> SMQSSKRSSRSVEDDKEGHLVCRIGDWLQERYEIVGNLGEGTFGKVVECLDHARGKSQVALKIIRNVGKYREAARLEINVLKKIKEKDKENKFLCVLMSDWFNFHGHMCIAFELLGKNTFEFLKENNFQPYPLPHVRHMAYQLCHALRFLHENQLTHTDLKPENILFVNSEFETLYNEHKSCEEKSVKNTSIRVADFGSATFDHEHHTTIVATRHYRPPEVILELGWAQPCDVWSIGCILFEYYRGFTLFQTHENREHLVMMEKILGPIPSHMIHRTRKQKYFYKGGLVWDENSSDGRYVK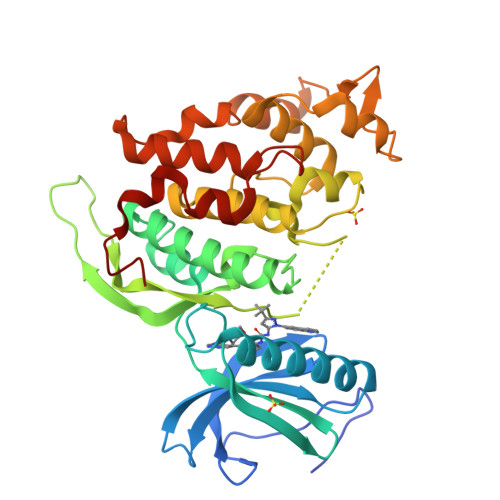ENCKPLKSYMLQDSLEHVQLFDLMRRMLEFDPAQRITLAEALLHPFFAGLTPEERSFHT> MKNISEDVIKYMPVTNKTIILDAGHGGIDPGALNKDKSTSEKDINLAITLKLRELIESSGG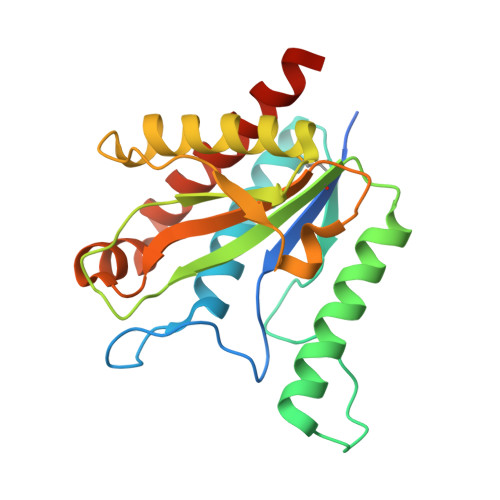LVILTREDDSSLYKEENNKTTRQKYNENLKNRKEIISNSNANMFVSIHLNAFEQSKYYGAQTFYPKDKQDSKELSKCIQEELKRVVDKTNNREVKPRDDIYLLKDNNIPSVLIECGFLSNEKECKLLTDETYQEKIAWAIYIGIQKYLSVDKLAAA> MSRAYDLVVLGAGSGGLEAGWNAAVTHKKKVAVVDVQATHGPPLFAALGGTCVNVGCVPKKLMVTGAQYMDLIRESGGFGWEMDRESLCPNWKTLIAAKNKVVNSINESYKSMFADTEGLSFHMGFGALQDAHTVVVRKSEDPHSDVLETLDTEYILIATGSWPTRLGVPGDEFCITSNEAFYLEDAPKRMLCVGGGYIAVEFAGIFNGYKPCGGYVDLCYRGDLILRGFDTEVRKSLTKQLGANGIRVRTNLNPTKITKNEDGSNHVHFNDGTEEDYDQVMLAIGRVPRSQALQLDKAGVRTGKNGAVQVDAYSKTSVDNIYAIGDVTNRVMLTPVAINEGAAFVETVFGGKPRATDHTKVACAVFSIPPIGTCGMTEEEAAKNYETVAVYASSFTPLMHNISGSKHKEFMIRIITNESNGEVLGVHMLGDSAPEIIQSVGICMKMGAKISDFHSTIGVHPTSAEELCSMRTPAYFYESGKRVEKLS

Leishmania uses trypanothione as its main detoxifying molecule, allowing the parasite to neutralize the reactive oxygen species produced by macrophages during the infection. Trypanothione is activated by Trypanothione reductase (TR), an enzyme that is absent in man but that is essential for parasite survival, and is therefore considered an attractive target. Trypanothione [N1,N8-bis(glutathionyl)spermidine] (TS2), which is synthesized by trypanothione synthetase (TryS) and reduced to T(SH)2 by the trypanothione reductase (TR), is used by the couple tryparedoxin/tryparedoxin peroxidase I (TXN/TXNPx) to neutralize hydrogen peroxide produced by macrophages during infection.[5–7] All attempts to date to obtain a TR-null mutant in L. donovani have failed and mutants displaying a partial trisomy of TR locus, where two TR alleles are disrupted by gene targeting, show attenuated infectivity and decreased ability to survive within the macrophages. The human homolog, glutathione reductase (hGR), that maintains glutathione in a reduced state, has a significantly different substrate binding site in terms of both volume and charge distribution, suggesting the possibility of identifying molecules able to selectively target TR.

We solved the X-ray structure of L. infantum TR in its oxidized state in complex with compound 3 (LiTR-3) at 3.37 Å resolution. The X-ray structure of the LiTR-compound 3 complex is homo-dimeric and is closely related to the TR-oxidized apo-form. However the Fo-Fc electron density map, allow the identification of the space occupied by the ligand and the residues involved in the binding even if the nitrophenyl group is not completely visible in the structure. In particular, as shown in Fig 8C, compound 3 is bound to the NADPH cavity entrance with an occupancy of 0.8, where it may form several mild electrostatic interactions with the protein residues lining its binding site. An electronic density peak was found close to Gly197, that has been interpreted as belonging to a sulfate ion (with 0.5 occupancy), which establishes electrostatic interactions with Gly197 and compound 3. Compound 3 is lined by Tyr221, Gly197, Asn254, Arg222 and Arg228 a residue which is electrostatically bound to Arg235 (NH1(Arg235)-NH2(Arg228) distance = 3.5 Å). Indeed, the superimposition between TR in oxidized state and the compound 3-TR complex shows that Arg228 and Arg222 undergo a 30° rotation (clockwise and anticlockwise, respectively) to allow compound binding. In particular, the nitro-phenyl group maps to the position of the adenine ring in the NADPH bound TR, and the two arginine residues (Arg222 and Arg228) that in the reduced enzyme interact with the adenine ribose phosphate moiety adopts a completely different conformation in the compound 3-TR complex. As shown by the structural analysis, residues Tyr221 and Asn254, which are involved in ligand binding to TR, are not conserved in hGR, where they are replaced by Ile217 and Gln250, respectively.>[2x]GQQPPLALPPPPPLPLPLPLPQPPPPQPPADEQPEPRTRRRAYLWCKE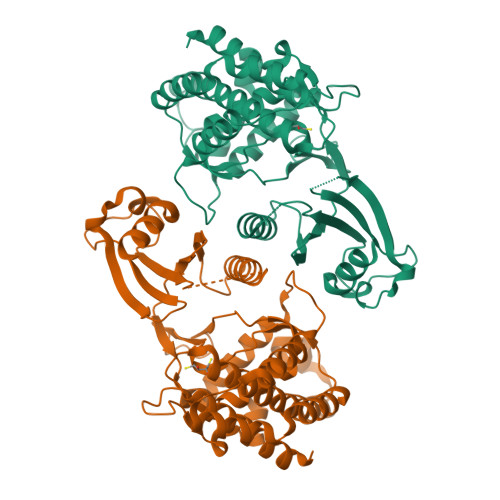FLPGAWRGLREDEFHISVIRGGLSNMLFQCSLPDTTATLGDEPRKVLLRLYGAILQVGAEAMVLESVMFAILAERSLGPKLYGIFPQGRLEQFIPSRRLDTEELSLPDISAEIAEKMATFHGMKMPFNKEPKWLFGTMEKYLKEVLRIKFTEESRIKKLHKLLSYNLPLELENLRSLLESTPSPVVFCHNDCQEGNILLLEGRENSEKQKLMLIDFEYSSYNYRGFDIGNHFCEWMYDYSYEKYPFFRANIRKYPTKKQQLHFISSYLPAFQNDFENLSTEEKSIIKEEMLLEVNRFALASHFLWGLWSIVQAKISSIEFGYMDYAQARFDAYFHQKRKLGV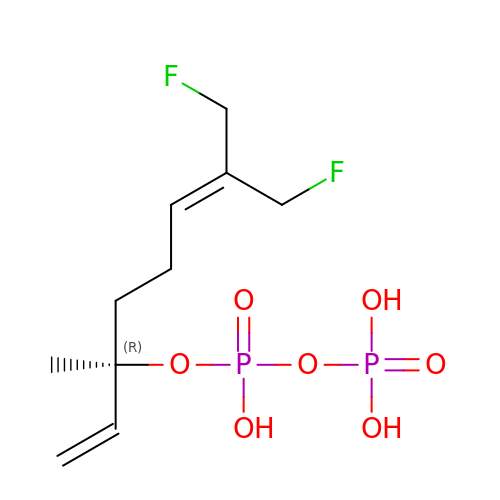(3R)-8-fluoro-7-(fluoromethyl)-3-methylocta-1,6-dien-3-yl trihydrogen diphosphate | C10 H18 F2 O7 P2 | POYBZGMZDXIMIL-JTQLQIEISA-N>[2x]MAEKVLVTGGAGYIGSHTVLELLEAGYLPVVIDNFHNAFRGGGSLPESLRRVQELTGRSVEFEEMDILDQGALQRLFKKYSFMAVIHFAGLKAMGESVQKPLDYYRVNLTGTIQLLEIMKAHGVKNLVFSSSATVYGNPQYLPLDE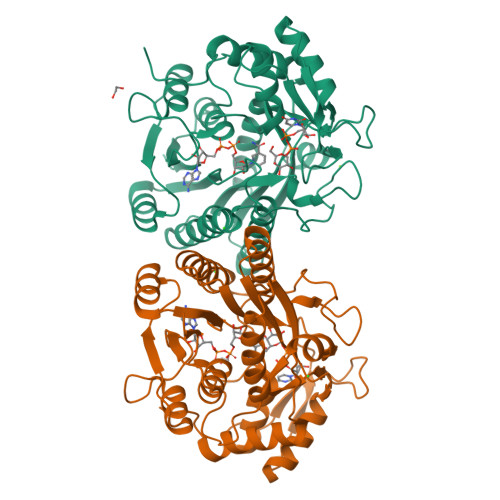AHPTGGCTNPYGKSKFFIEEMIRDLCQADKTWNVVLLRYFNPTGAHASGCIGEDPQGIPNNLMPYVSQVAIGRREALNVFGNDYDTEDGTGVRDYIHVVDLAKGHIAALRKLKEQCGCRIYNLGTGTGYSVLQMVQAMEKASGKKIPYKVVARREGDVAACYANPSLAQEELGWTAALGLDRMCEDLWRWQKQNPSGFGTQA> MDQQGMVKKRLAVLVGCN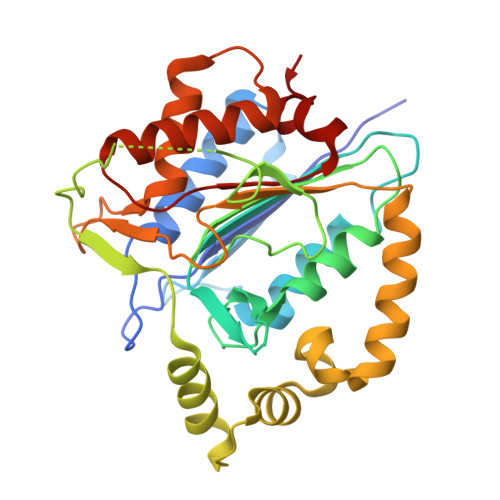YPNTRNELHGCINDVLAMKETILSRFGFKQDDIEVLTDEPESKVKPTGANIKAALRRMVDKAQAGSGDILFFHYSGHGTRIPSVKSAHPFKQDEAIVPCDFNLITDVDFRELVNQLPKGTSFTMISDSGHSGGLIDKEKEQIGPSSVSSNISPAIETTNKTITSRALPFKAVLDHLSSLTGITTSDIGTHLLELFGRDAGLKFRLPAMDLMDLLETMTAREKHVDSGILMSGCQADETSADVGVGNGKAYGAFSNAIQRVLNENEGAMKNKQLVMMARDVLERLGFHQHPCLYCSDQNADATFLSQP>[4x]MR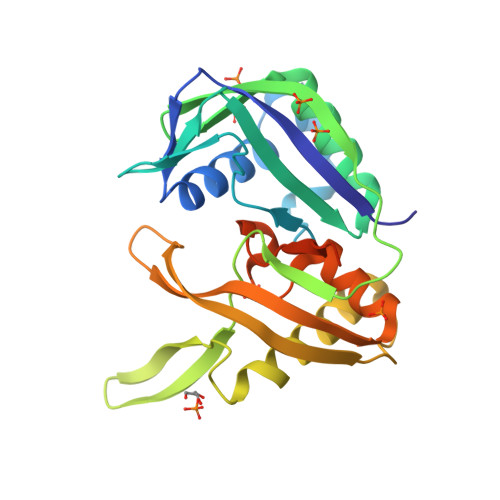ESMRIELELQTDNFTVIPYNHQYYLASAIYNKIHSANPAYAKRLHNYQKFKFFTFSLLQIRKRVIRKEGIETIDGKAYLYISSPNNEFIENFVAGLLEDGKLRVGNVEFFVRKAKILPIPKKFNILKTISPIYLKTMIETEDGLKTYDLLPNNSKFYENLKNNLKKKYEAFYNEKCDMNFEFEVLKFRPKRMRIKNDIYCRCSEMVFKVWGDYDLIKFGYECGFGEKNSMGFGMVVNVEDKNQKNKKLKTKILEHHHHHH β-Propeller proteins are common natural disc-like pseudo-symmetric proteins that contain multiple repeats (‘blades’) each consisting of a 4-stranded anti-parallel β-sheet. In the larger propellers a so-called “Velcro closure” is found, in which the N- and C-terminal β-strands are part of the same β-sheet, keeping the propeller closed. This “Velcro” can occur in different positions; in the “Velcro 1-3” variant, the closing β-sheet consists of one N-terminal and three C-terminal strands, while for the “Velcro 3-1” variant, the opposite is true. Starting from a highly repetitive β-propeller sequence, we designed a consensus motif sequence that formed a perfectly symmetric 7-bladed β-propeller.

All the WRAP-T permutants expressed well and could be purified easily. Solving the crystal structures revealed that they possess an identical structure. Interestingly, the different position of the chain termini had an influence on the preferred crystallisation conditions and crystal packing. While for previously designed symmetric proteins, the proteins typically packed in distinct symmetric ways reflecting the inherent six-, eight- or nine-fold symmetry of the proteins, here no clear symmetric interactions could be observed within the lattice. This may be expected given the incompatibility of seven-fold internal symmetry with any space group. Despite the non-equivalent positions of each blade within the crystal structures, the proteins proved to be perfectly symmetric, with a TM-score above 0.97 calculated by CE-symm. Analysing the thermal and chemical stability of the WRAP-T permutants revealed that nvWRAP-T, lacking the velcro closure, is just as stable as the variant v13WRAP-T. While v31WRAP-T is considerably more resistant to GdnHCl induced denaturation compared to the other proteins, its increased thermal stability is not that significant. A striking difference however is the stability of the “non-Velcro” variant, the least stable for Pizza but as stable as the natural “Velcro” position in WRAP-T. This may be due to differences between the sequences, as the two different “non-Velcro” variants of Pizza have different stabilities as well.

>[2x]MGHSSSVTGVAFSPDGQTIASASDDKTVKLWNRNGQLLQTLTGHSSSVTGVAFSPDGQTIASASDDKTVKLWNRNGQLLQTLTGHSSSVTGVAFSPDGQTIASASDDKTVKLWNRNGQLLQTLTGHSSSVTGVAFSPDGQTIASASDDKTVKLWNRNGQLLQTLTGHSSSVTGVAFSPDGQTIASASDDKTVKLWNRNGQLLQTLTGHSSSVTGVAFSPDGQTIASASDDKTVKLWNRNGQLLQTLTGHSSSVTGVAFSPDGQTIASASDDKTVKLWNRNGQLLQTLTGHSSSVTGVAFSPDGQTIASASDDKTVKLWNRNGQLLQTLT NADPH oxidase 5 (NOX5) catalyzes the production of superoxide free radicals and regulates physiological processes from sperm motility to cardiac rhythm. NOX5 catalyzes the electron transfer from cytosolic NADPH to extracellular oxygen to produce superoxide (O2-) in the presence of intracellular Ca2+ ions. Like DUOX1-2, Ca2+ activates NOX5 by binding to its regulatory EF-hand domain (EFD). Each protomer contains a catalytic core with TMD, FBD and NBD and a regulatory EFD.

Focused refinement followed by symmetry expansion was performed to improve the local resolution of cytosolic domain of NOX5 in the pre-reaction state. Here we first use the pre-reaction state to describe the overall structure of NOX5. NOX5 forms homodimers rather than homotetramers as previously reported. Briefly, the TMD contains six transmembrane helices (TM1–6) and binds two heme molecules, and the cytosolic DHD binds FAD and NADPH. In the pre-reaction state, EF1 and EF2 have a low local resolution, which only allows the assignment of secondary structures. Part of INS1 displayed a helical density that should belong to PhosR, extending from the FBD and packed against the EFD. We observed a helix from the PhosR motif in the pre-reaction structure but not intermediate state 3 structure, docking against a negatively charged surface on the EFD. PhosR may stabilize the EFD in the inactive state, but this motif is released upon phosphorylation, facilitating the transition of the EFD to active conformations. Instead, the corresponding residue, Val362 and three other residues (Cys235, Val275 and Leu332) are located between the two hemes and might contribute to electron transfer. The distance between NADPH and FAD, which is >10 Å, is not optimal for transferring electrons, as NADPH and FAD are solvent-exposed.

>[2x]MSAEEDARWLRWVTQQFKTIAGEDGEISLQEFKAALHVKESFFAERFFALFDSDRSGTITLQELQEALTLLIHGSPMDKLKFLFQVYDIDGSGSIDPDELRTVLQSCLRESAISLPDEKLDQLTLALFESADADGNGAITFEELRDELQRFPGVMENLTISAAHWLTAPAPRPRPRRPRQLTRAYWHNHRSQLFCLATYAGLHVLLFGLAASAHRDLGASVMVAKGCGQCLNFDCSFIAVLMLRRCLTWLRATWLAQVLPLDQNIQFHQLMGYVVVGLSLVHTVAHTVNFVLQAQAEASPFQFWELLLTTRPGIGWVHGSASPTGVALLLLLLLMFICSSSCIRRSGHFEVFYWTHLSYLLVWLLLIFHGPNFWKWLLVPGILFFLEKAIGLAVSRMAAVCIMEVNLLPSKVTHLLIKRPPFFHYRPGDYLYLNIPTIARYEWHPFTISSAPEQKDTIWLHIRSQGQWTNRLYESFKASDPLGRGSKRLSRSVTMRKSQRSSKGSEILLEKHKFCNIKCYIDGPYGTPTRRIFASEHAVLIGAGIGITPFASILQSIMYRHQKRKHTCPSCQHSWIEGVQDNMKLHKVDFIWINRDQRSFEWFVSLLTKLEMDQAEEAQYGRFLELHMYMTSALGKNDMKAIGLQMALDLLANKEKKDSITGLQTRTQPGRPDWSKVFQKVAAEKKGKVQVFFCGSPALAKVLKGHCEKFGFRFFQENF;>[2x]AAAAAAAAAAAAA1-(9~{H}-fluoren-9-yl)-3-(2-methyl-4-phenyl-pyrimidin-5-yl)urea | C25 H20 N4 O | 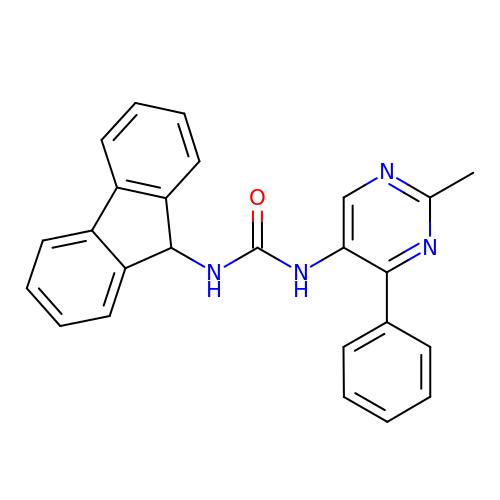PKOROKYRNIDSPX-UHFFFAOYSA-N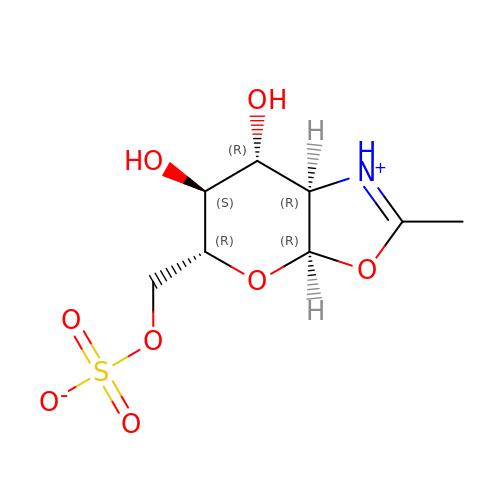[(3~{a}~{R},5~{R},6~{S},7~{R},7~{a}~{R})-2-methyl-6,7-bis(oxidanyl)-5,6,7,7~{a}-tetrahydro-3~{a}~{H}-pyrano[3,2-d][1,3]oxazol-1-ium-5-yl]methyl sulfate | C8 H13 N O8 S | JTXHTZSXIURMTP-PVFLNQBWSA-N> AQVSRQNYFNINYFKDAASNG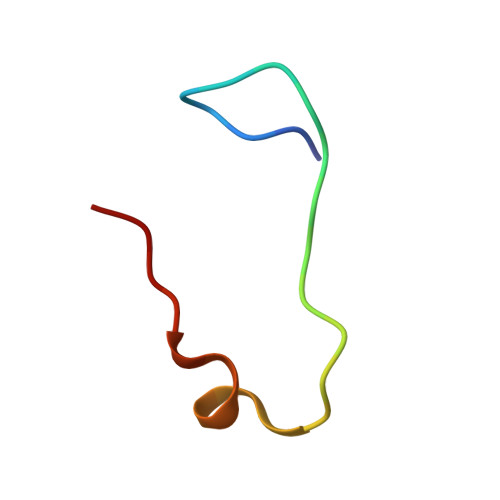ASKL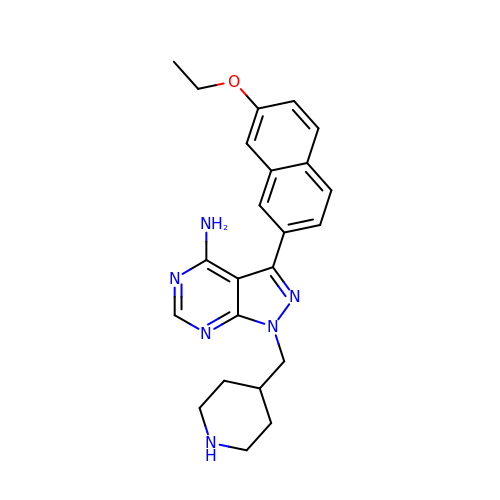3-(7-ethoxynaphthalen-2-yl)-1-(piperidin-4-ylmethyl)-1H-pyrazolo[3,4-d]pyrimidin-4-amine | C23 H26 N6 O | KMHCRQINFJTBPW-UHFFFAOYSA-N> AFVVTDNCIK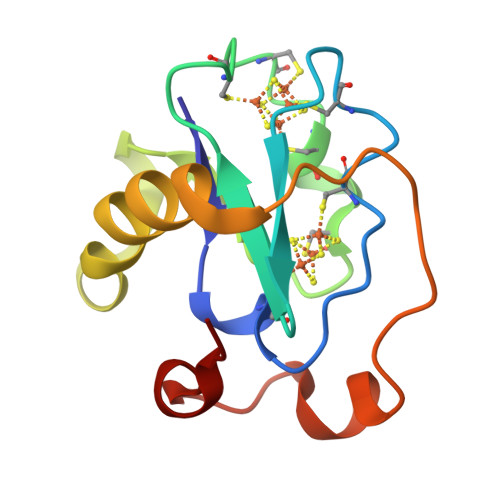CKYTECVEVCPVDCFYEGPNFLVIHPDECIDCALCEPECPAQAIFSEDEVPEDMQEFIQLNAELAEVWPNITEKKDPLPDAEDWDGVKGKLQHLER> MAHIFVKPELVAEIGVKQLQREIVLPGLVWTNPLTDFGGSKNDTITVRVPAITTANRRDLRDPDRTVIASELVEHSFGVTLDKHVYAALKFTDEQRTLDIRDYTKQVLMPQVSAVAYELEDYIAELIEGAPYEETILIDPADTVPAFITADQRMGEANVPTDS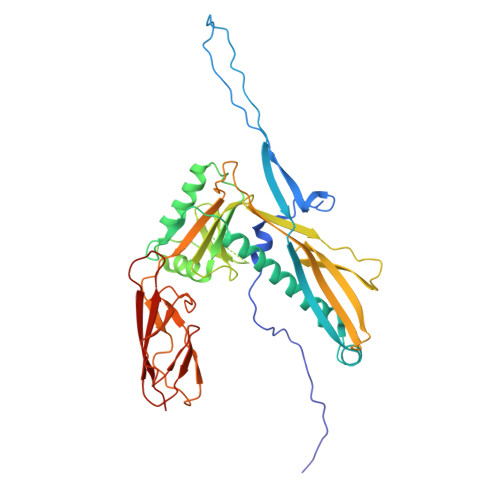RRLVVGSAVAAALAKDKQFRHADWSGDQANAALREAHVGRLAGMNVIRSNAIAPDKAYLWHRTAFILAYRTPVVPEGAKAGASFSANGVALRWLADYDYSQLGDRTLLDVFTGRKVVTEVDGSFVRAVELQLQASSITIVGGAFALATTTGTKQLKVRDDNGTDVTARCTFASSAGTKATVSAAGLVTGVAAGTADITASYVPPQGGTAKTATVTVTVP> SMGDDCFSLRRCCLPQPGETSNLIIMRGARASPRTLNLSQLSFHRVDQKEITQLSHLGQGTRTNVYEGRLRVEGSGDPEEGKMDDEDPLVPGRDRGQELRVVLKVLDPSHHDIALAFYETASLMSQVSHTHLAFVHGVCVRGPENIMVTEYVEHGPLDVWLRRERGHVPMAWKMVVAQQLASALSYLENKNLVHGNVCGRNILLARLGLAEGTSPFIKLSDPGVGLGALSREERVERIPWLAPECLPGGANSLSTAMDKWGFGATLLEICFDGEAPLQSRSPSEKEHFYQRQHRLPEPSCPQLATLTSQCLTYEPT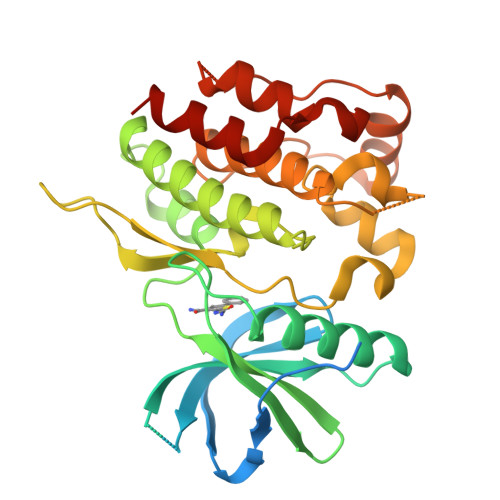QRPSFRTILRDLTRLQPHN>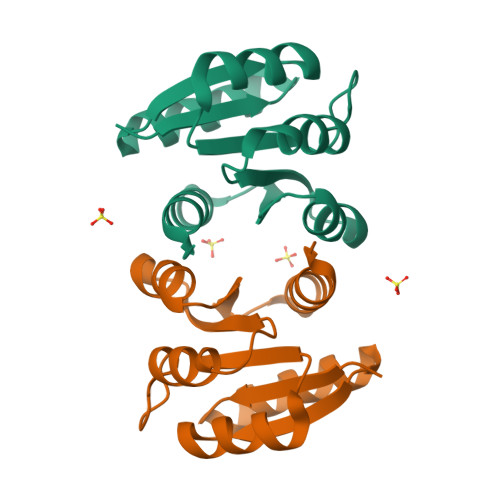[2x]MDKKILVVDDEKPIADILEFNLRKEGYEVHCAHDGNEAVEMVEELQPDLILLDIMLPNKDGVEVCREVRKKYDMPIIMLTAKDSEIDKVIGLEIGADDYVTKPFSTRELLARVKANLRRQLTLEHHHHHH> MHVAQPAVVLASSRGIASFVCEYASPGKATEVRVTVLRQADSQVTEVC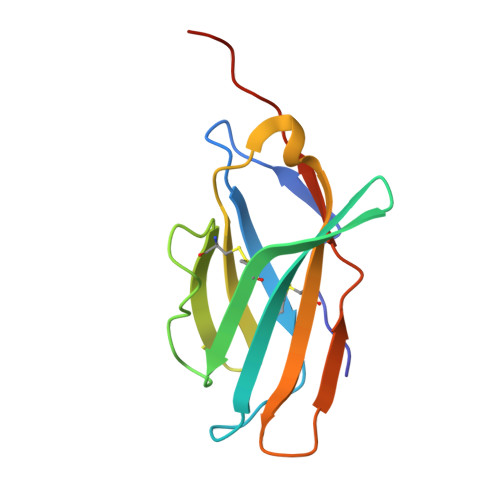AATYMMGNELTFLDDSICTGTSSGNQVNLTIQGLRAMDTGLYICKVELMYPPPYYLGIGNGTQIYVIDPEPCPDSD Cep104 is a key factor involved in cilia formation and length regulation that rides on the ends of elongating and shrinking cilia. It is mutated in Joubert syndrome, a genetically heterogeneous ciliopathy. Here we provide structural and biochemical data that Cep104 contains a tubulin-binding TOG (tumor overexpressed gene) domain and a novel C2HC zinc finger array. We have structurally characterized two of these domains, a central tubulin-binding TOG (tumor overexpressed gene) domain and a C-terminal domain consisting of an array of four Zn fingers (ZNF domain).

However, we obtained crystals for the human apo-Cep104 ZNF domain (S763E mutant) and solved its structure by X-ray crystallography to a resolution of 1.8 Å. The S763E mutation was used since we found it to improve the solubility of the protein. The residue S763 is located at the loop connecting the β hairpin to the α helix of the first ZNF. The Cep104 ZNF structure consists of four tandem C2HC Zn fingers that pack together to form a single globular domain that, to our knowledge, represents a novel, previously unobserved arrangement of Zn fingers. The individual Zn fingers are variants of the classical C2H2 ZNFs in which the last Zn-coordinating residue is Cys instead of His. They consist of a β hairpin followed by an α helix that packs on it. The Zn ion is coordinated by two Cys residues located on the hairpin and by His and Cys residues from the helix with the exception of ZNF3 and ZNF4, in which the last Zn-coordinating Cys is located at a loop region downstream of the C-terminal helix cap (left). In the Cep104 domain, the sequence separation between the individual ZNFs is variable and increases from two residues between ZNF1 and ZNF2 to eight residues between ZNF3 and ZNF4. The strict conservation of these residues suggests that the compact globular shape of this domain is not due to crystal packing but that the four C2HC Cep104 ZNFs probably function as an integral, single unit. Consistent with this notion is that this domain shows a continuous patch of surface conservation that probably constitutes a protein-protein interaction interface for its binding partners.

>[4x]GPHMDEHYLDNLCIFCGERSEEFTEEGLDLHYWKHCLMLTRCDHCKQVVEISSLTEHLLTECDKKDGFGKCYRCSEAVFKEELPRHIKHKDCNPAKPEKLANRCPLCHENFSPGEEAWKAHLMGPAGCTMNLRK> RETHLRSILHTIPDAMIVIDGHGIIQLFSTAAERLFG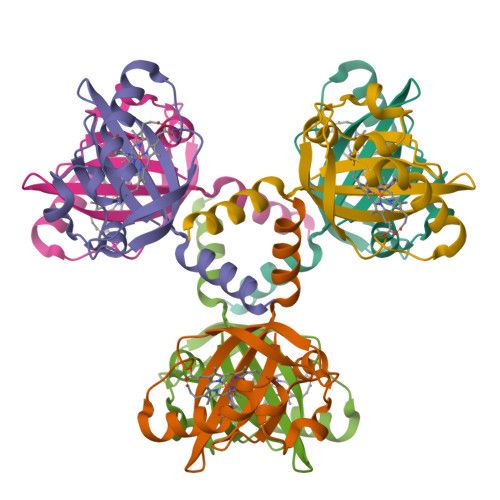WSELEAIGQNVNILMPEPDRSRHDSYISAYRTTSDPHIIGIGRIVTGKRRDGTTFPMHLSIGEMQSGGEPYFTGFVRDLTEHQQTQARLQELQ>ADKLFINALKKKFEESPEEKKTTFYTLGGWKQSERKTEFVNAGKEVAAKRGIPQYNPDIGTPLGQRVLMPYQVSTTDTYVEGDDLHFVNNAAMQQMWDDIRRTVIVGLNHAHAVIEKRLGKEVTPETITHYLETVNHAMPGAAVVQEHMVETHPALVADSYVKVFTGNDEIADEIDPAFVIDINKQFPEDQAETLKAEVGDGIWQVVRIPTIVSRTCDGATTSRWSAMQIGMSMISAYKQAAGEAATGDFAYAAKHAEVIHMGTYLPVRRARGENEPGGVPFGYLADICQSSRVNYEDPVRVSLDVVATGAMLYDQIWLGSYMSGGVGFTQYATAAYTDNILDDFTYFGKEYVEDKYGLCEAPNNMDTVLDVATEVTFYGLEQYEEYPALLEDQFGGSQRAAVVAAAAGCSTAFATGNAQTGLSGWYLSMYLHKEQHSRLGFYGYDLQDQCGASNVFSIRGDEGLPLELRGPNYPNYAMNVGHQGEYAGISQAPHAARGDAFVFNPLVKIAFADDNLVFDFTNVRGEFAKGALREFEPAGERALITPA[2x];>[2x]AKFEDKVDLYDDRGNLVEEQVPLEALSPLRNPAIKSIVQGIKRTVAVNLEGIENALKTAKVGGPACKIMGRELDLDIVGNAESIAAAAKEMIQVTEDDDTNVELLGGGKRALVQVPSARFDVAAEYSAAPLVTATAFVQAIINEFDVSMYDANMVKAAVLGRYPQSVEYMGANIATMLDIPQKLEGPGYALRNIMVNHVVAATLKNTLQAAALSTILEQTAMFEMGDAVGAFERMHLLGLAYQGMNADNLVFDLVKANGKEGTVGSVIADLVERALEDGVI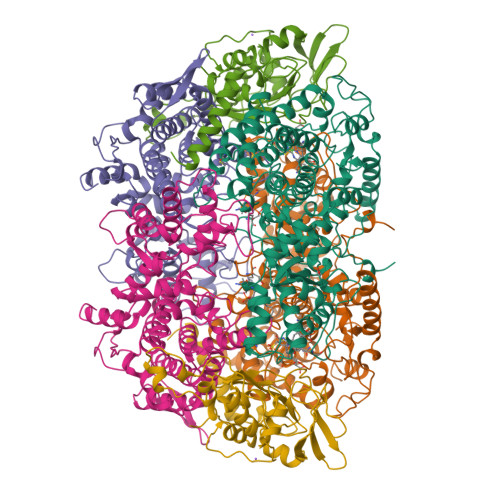KVEKELTDYKVYGTDDLAMWNAYAAAGLMAATMVNQGAARAAQGVSSTLLYYNDLIEFETGLPSVDFGKVEGTAVGFSFFSHSIYGGGGPGIFNGNHIVTRHSKGFAIPCVAAAMALDAGTQMFSPEATSGLIKEVFSQVDEFREPLKYVVEAAAEIKNEI;>[2x]AQYYPGTTKVAQNRRNFCNPEYELEKLREISDEDVVKILGHRAPGEEYPSVHPPLEEMDEPEDAIREMVEPIDGAKAGDRVRYIQFTDSMYFAPAQPYVRSRAYLCRYRGADAGTLSGRQIIETRERDLEKISKELLETEFFDPARSGVRGKSVHGHSLRLDEDGMMFDMLRRQIYNKDTGRVEMVKNQIGDELDEPVDLGEPLDEETLMEKTTIYRVDGEAYRDDVEAVEIMQRIHVLRSQGGFNL>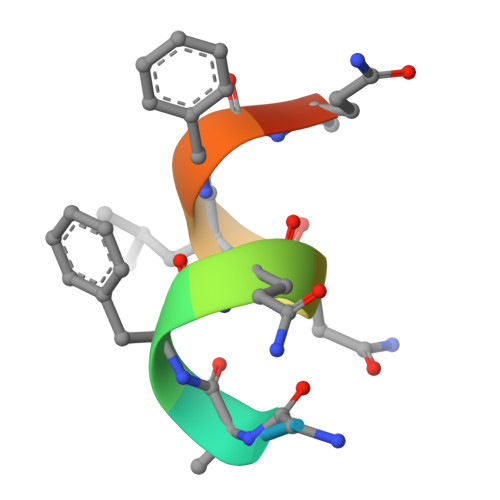 RGAFQNLFQSV> MASSRSELLLDRFAEKIGVGSISFNENRLCSFAIDEIYYISLSDANDEYMMIYGVCGKFPTDN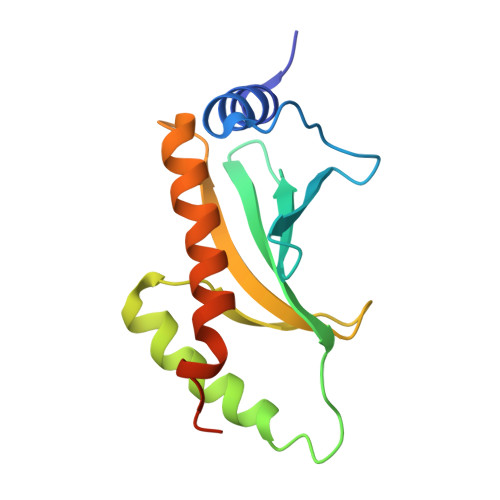PNFALEILNANLWFAENGGPYLCYESGAQSLLLALRFPLDDATPEKLENEIEVVVKSMENLYLVLHNQGITLENEH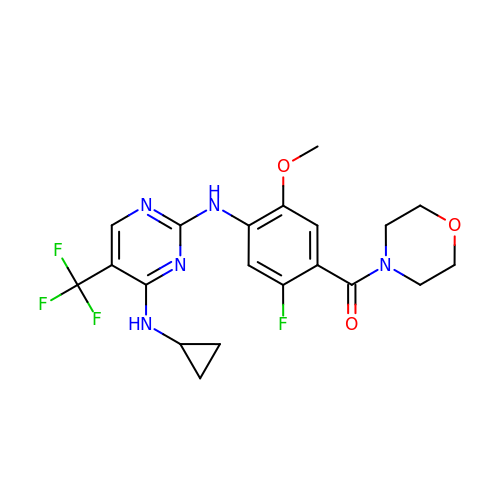(4-{[4-(cyclopropylamino)-5-(trifluoromethyl)pyrimidin-2-yl]amino}-2-fluoro-5-methoxyphenyl)(morpholin-4-yl)methanone | C20 H21 F4 N5 O3 | FKNAWDCGDQUZRV-UHFFFAOYSA-N> SITKTELDGILPLVARGKVRDIYEVDAGTLLFVATDRISAYDVIMENSIPEKGILLTKLSEFWFKFLSNDVRNHLVDIAPGKTIFDYLPAKLSEPKYKTQLEDRSLLVHKHKLIPLEVIVRGYITGSAWKEYVKTGTVHGLKQPQGLKESQEFPEPIFTPSTKAEQGEHDENISPAQAAELVGEDLSRRVAELAVKLYSKCKDYAKEKGIIIADTKFEFGIDEKTNEIILVDEVLTPDSSRFWNGASYKVGESQDSYDKQFLRDWLTANKLNGVNGVKMPQDIVDRTRAKYI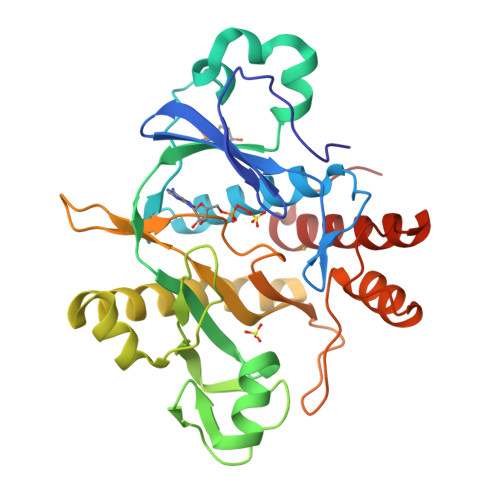EAYETLTGSKWSH> GTTVHCDYLNRPHKSIHRRRTDPMVTLSSILESIINDMRDLPNTYPFHTPVNAKVVKDYYKIITRPMDLQTLRENVRKRLYPSREEFREHLELIVKNSATYNGPKHSLTQISQSMLDLCDEKLKEKEDKLARLEKAINPLLDDDDQVAFSFILDNIVTQKMMAVPDSWPFHHPVNK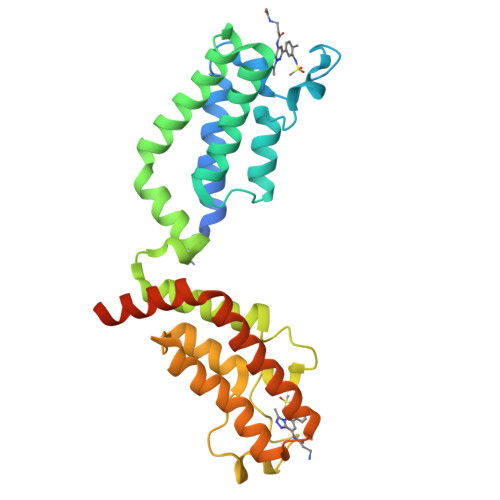KFVPDYYKVIVNPMDLETIRKNISKHKYQSRESFLDDVNLILANSVKYNGPESQYTKTAQEIVNVCYQTLTEYDEHLTQLEKDICTAKEAALEEAELESLDPMT>[4x]MKAAAKRISDGVYWTGVLDWDLRNYHGYTLQGTTYNAYLVCGDEGVALIDNSYPGTFDELMARVEDALQQVGMERVDYIIQNHVEKDHSGVLVELHRRFPEAPIYCTEVAVKGLLKHYPSLREAEFMTVKTGDVLDLGGKTLTFLETPLLHWPDSMFTLLDEDGILFSNDAFGQHLCCPQRLDREIPEYILMDAARKFYANLITPLSKLVLKK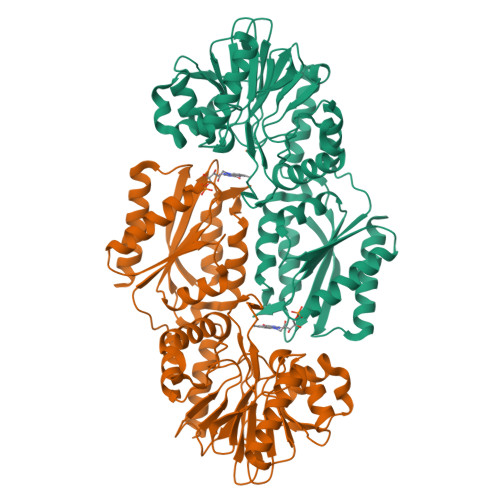FDEVKELGLLERIQMIAPSHGQIWTDPMKIIEAYTGWATGMVDERVTVIYDTMHGSTRKMAHAIAEGAMSEGVDVRVYCLHEDDRSEIVKDILESGAIALGAPTIYDEPYPSVGDLLMYLRGLKFNRTLTRKALVFGSMGGNGGATGTMKELLAEAGFDVACEEEVYYVPTGDELDACFEAGRKLAAEIRR N-hydroxycyclopent-1-ene-1-carboxamide | C6 H9 N O2 | 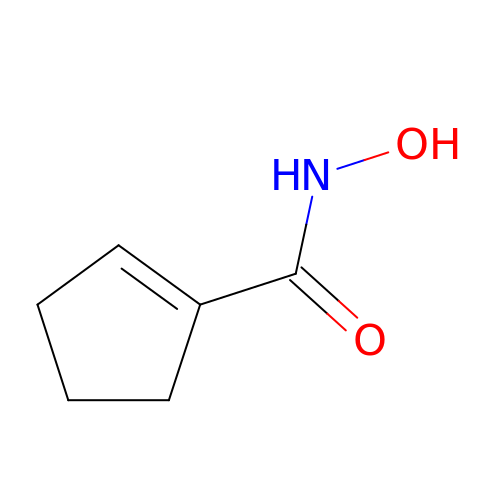RYYGSXXWQSXKRP-UHFFFAOYSA-N>MPSETPQAEVGPTGCPHRSGPHSAKGSLEKGSPEDKEAKEPLWIRPDAPSRCTWQLGRPASESPHHHTAPAKSPKILPDILKKIGDTPMVRINKIGKKFGLKCELLAKCEFFNAGGSVKDRISLRMIEDAERDGTLKPGDTIIEPTSGNTGIGLALAAAVRGYRCIIVMPEKMSSEKVDVLRALGAEIVRTPTNARFDSPESHVGVAWRLKNEIPNSHILDQYRNASNPLAHYDTTADEILQQCDGKLDMLVASVGTGGTITGIARKLKEKCPGCRIIGVDPEGSILAEPEELNQTEQTTYEVEGIGYDFIPTVLDRTVVDKWFKSNDEEAFTFARMLIAQEGLLCGGSAGSTVAVAVKAAQELQEGQRCVVILPDSVRNYMTKFLSDRWMLQKGFLKEEDLTEKKPWWWHLRVQELGLSAPLTVLPTITCGHTIEILREKGFDQAPVVDEAGVILGMVTLGNMLSSLLAGKVQPSDQVGKVIYKQFKQIRLTDTLGRLSHILEMDHFALVVHE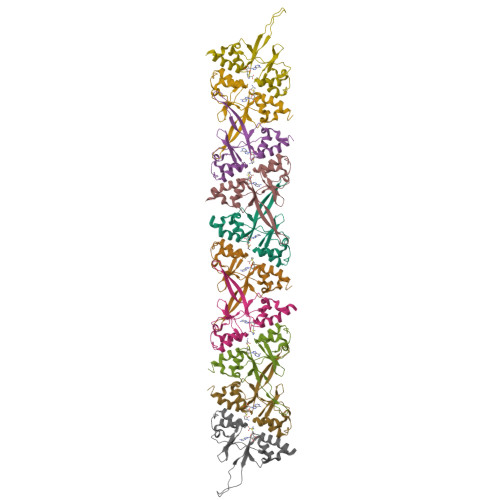QIQYHSTGKSSQRQMVFGVVTAIDLLNFVAAQERDQKAAHHHHHH[10x]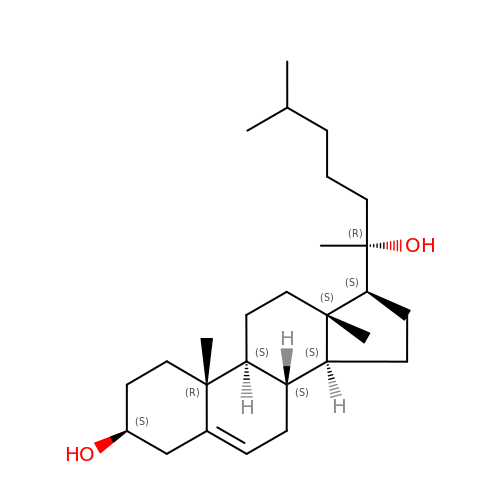20-HYDROXYCHOLESTEROL | C27 H46 O2 | MCKLJFJEQRYRQT-MGNSQDQZSA-N CCs are quaternary structures comprising two or more α-helices supercoiled around each other with cyclic (Cn) or dihedral (Dn) symmetry. Here, we describe variants with all combinations of the aliphatic residues, Ile, Leu and Val, at a and d to give four classes of peptide: the ββ class, with a and d = Ile or Val; Lβ, a = Leu and d = Ile or Val; βL, a = Ile or Val and d = Leu; and LL, a = d = Leu. Peptides are named systematically appending the one-letter code for the amino acids at the a and d sites to “CC-Type2-“; e.g., CC-Hept becomes CC-Type2-LI. In summary, solution-phase data and X-ray crystal structures demonstrate conclusively that different classes of Type-2 coiled-coil (CC) peptides—i.e., based on abcdefg repeats with predominantly hydrophobic residues at a, d, e and g—adopt a range of distinct states.

Not all of the peptides with e = g = Ala were soluble, therefore, some were made with g = Ser or Glu, and suffixes “-Sg” or “-Eg” are added to the systematic names. By contrast, those of the βL class and peptide CC-Type2-LL showed weak or non-specific binding of DPH. In addition, we found hitherto unreported plasticity in the βL class of structures: compared with CC-Type2-IL-Eg, CC-Type2-IL-Sg—which differ at peripheral g and c sites—is a fully collapsed CC structure above tetramer. The latter makes an incomplete slipped barrel of five helices with a sixth helix packed against these to fill the void completely and consolidate a hydrophobic core; i.e., screw symmetry is broken in this structure. The two collapsed structures were more complicated. Nonetheless, both had extensive KIH interfaces linking all helices and, as such, are CC-based structures. CC-Type2-IL-Sg only had identity symmetry element (E) due to a Type-3 interfaced helix docking into a slipped barrel architecture, Fig. 4a. Sequences with β-branched (Ile or Val) residues at both a and d or with Leu at a plus Ile at d (ββ and LI classes, respectively) form cyclically symmetric, blunt-ended structures with central channels, i.e., they are α-helical barrels. βL class peptides adopt slipped barrel-like or collapsed structures depending on the amino acid at g.

>[18x]XGELAQSIKELAKSIKELAWSIKELAQSIKGX> DPDQFRAIIESPEGAGHVGYQYRRNTGSTMRMVSDVLDERVSLWDFHCDPSGNVIQPGPNVDSRQYLQAAIDYVSSNGGGTITIPAGYTWYLGSYGVGGIAGHSGIIQLRSNVNLNIEGRIHLSPFFDLKPFQVFVGFDNGDPASSGNLENCHIYGHGVVDFGGYEFGASSQLRNGVAFGRSYNCSVTGITFQNGDVTWAITLGWNGYGSNCYVRKCRFINLVNSSVNADHSTVYVNCPYSGVESCYFSMSSSFARNIACSVQLHQHDTFYRGSTVNGYCRGAYVVMHAAEAAGAGSYAYNMQVENNIAVIYGQFVILGSDVTATVSGHLNDVIVSGNIVSIGERAAFSAPFGAFIDIGPSGASNVQDIQRVLVTGNSFYAPANITDSAAITLRANLNGCTFIANNFDCRYMVYNAPGTTSPVVQNLVWDKSNVIGGTHANQRAGQNLFDMQFASVVNSTIEVQLSCEDLSMFSCILFPASCQLSYSKITVDSAWTKSMSNTAVFEGNQQAGANVYVSYPATVNLTS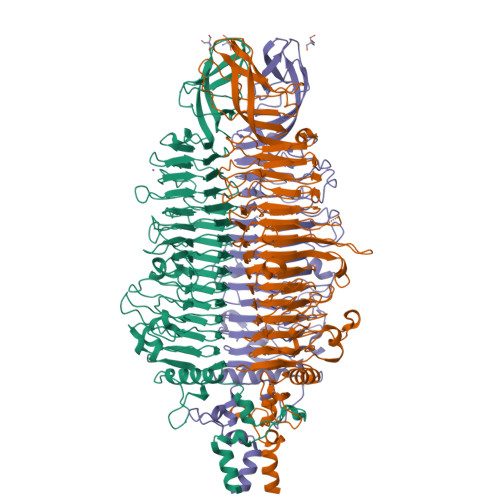YNTQGAVPFFSTDTNYAWVTSAYSLSINENLDFSPPATYTNKANGQLVGVGYNEIGGVRSVSVRLMLQRQV2,2-dimethyl-N-[(6-methyl-5-{[2-(1-methyl-1H-pyrazol-4-yl)pyridin-4-yl]oxy}pyridin-2-yl)carbamoyl]propanamide | C21 H24 N6 O3 | 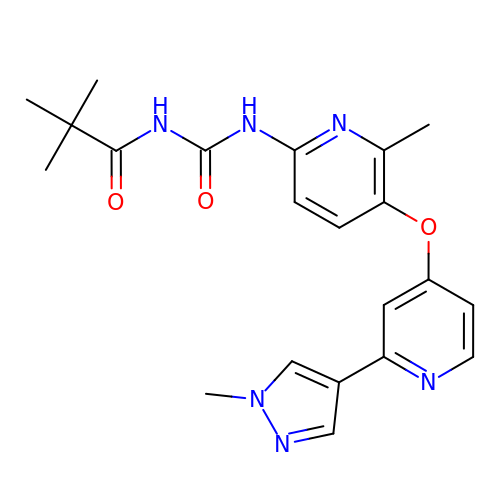WYLCQKJYTVNVCY-UHFFFAOYSA-N>GSRADFFTYETPKVIVVKSWTIGIINRVVQLLIISYFVGWVFLHEKAYQVRDTAIESSVVTKVKGSGLYANRVMDVSDYVTPPQG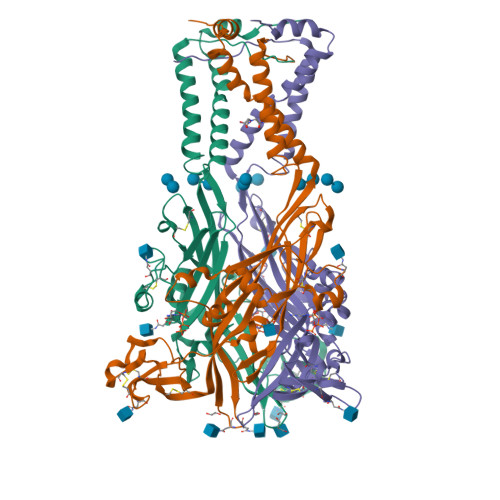TSVFVIITKMIVTENQMQGFCPESEEKYRCVSDSQCGPERLPGGGILTGRCVNYSSVLRTCEIQGWCPTEVDTVETPIMMEAENFTIFIKNSIRFPLFNFEKGNLLPNLTARDMKTCRFHPDKDPFCPILRVGDVVKFAGQDFAKLARTGGVLGIKIGWVCDLDKAWDQCIPKYSFTRLDSVSEKSSVSPGYNFRFAKYYKMENGSEYRTLLKAFGIRFDVLVYGNAGKFNIIPTIISSVAAFTSVGVGTVLCDIILLNFLKGADQYKAKKFEEVNET[2x]> GRRGVLMTL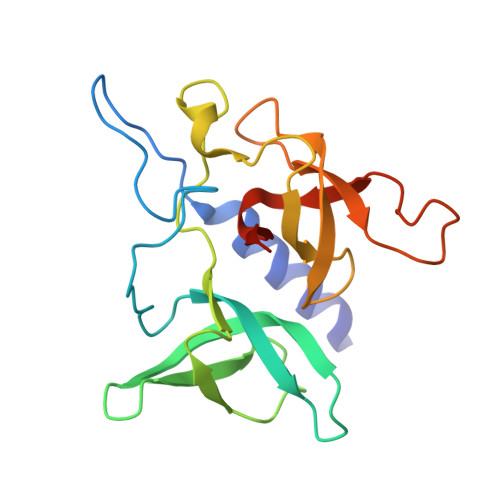LQQSAMTLPLWIGKPGDKPPPLCGAIPASGDYVARPGDKVAARVKAVDGDEQWILAEVVSYSHATNKYEVDDIDEEGKERHTLSRRRVIPLPQWKANPETDPEALFQKEQLVLALYPQTTCFYRALIHAPPQRPQDDYSVLFEDTSYADGYSPPLNVAQRYVVACKEPKKK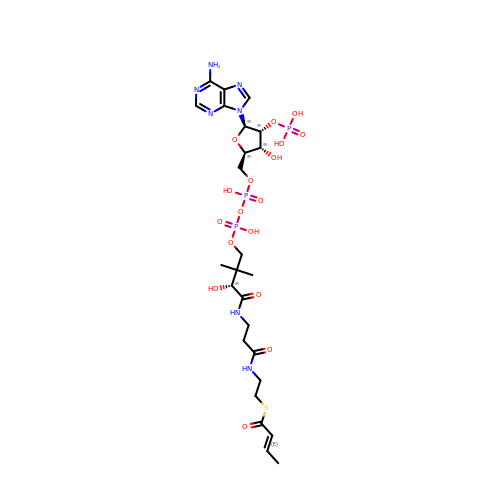S-{(9R,13R,15S)-17-[(2R,3R,4R,5R)-5-(6-amino-9H-purin-9-yl)-3-hydroxy-4-(phosphonooxy)tetrahydrofuran-2-yl]-9,13,15-trihydroxy-10,10-dimethyl-13,15-dioxido-4,8-dioxo-12,14,16-trioxa-3,7-diaza-13,15-diphosphaheptadec-1-yl}(2E)-but-2-enethioate | C25 H40 N7 O17 P3 S | BOZMQGABFDQJEL-PAXLJYGASA-N2,2'-oxydi(ethyn-1-ol) 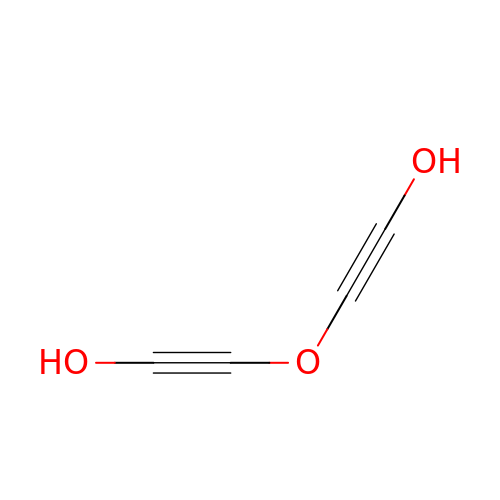| C4 H2 O3 | QFHUYNIAGZXZMU-UHFFFAOYSA-N> SGKAVDGNTLVLTEEFGLVKIKELYEKLDGKGRKTVEGNEEWTELETPVTVYGYRNGRIVGIKATHIYKGISSGMIEIRTRTGRKIKV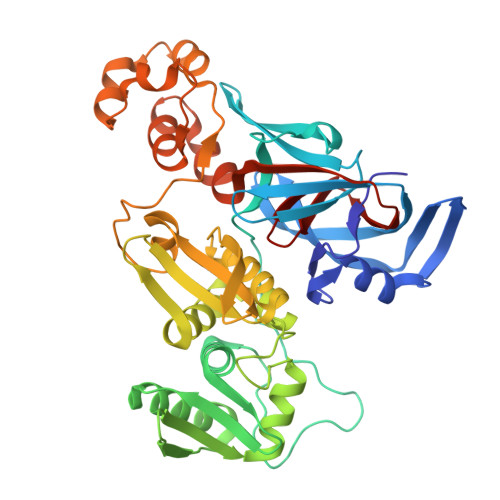TPIHKLFTGRVTKDGLALEEVMAMHIKPGDRIAVVKKIDGGEYVKLTTSPDFRKSRKIKVPEVLDEDLAEFLGYLIADGTLKPRTVAIYNNDESLLKRANFLSTKLFGINGKIVQERTVKALLIHSKPLVDFFRKLGIPESKKARNWKVPRELLLSPPSVVKAFINAYIVCDGYYHERKGEIEITTASEEGAYGLSYLLAKLGIYATFRKKQIKGKEYYRIAISGKTNLEKLGIKRETRGYTNIDIVPVEVESIYNALGRPYSELKGEGIEIHNYLNGENMTYETFRKFAKLVGLEEVAENHLKHILFDEVVEVKYIPEPQEVYDITTETHNFVGGNMPTLLHN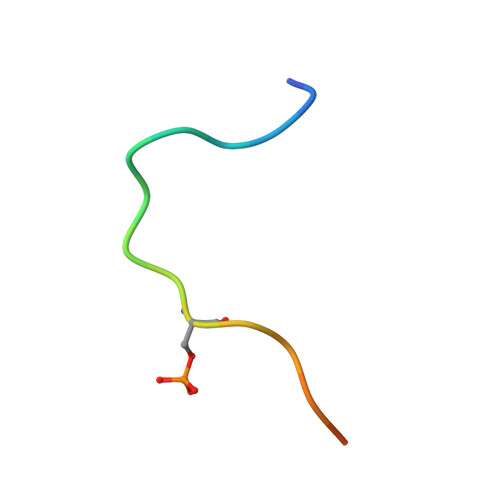> SGCFEDLAISASTSLGWG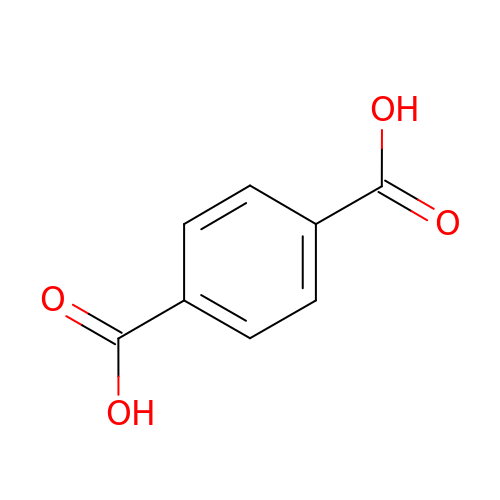terephthalic acid | C8 H6 O4 | KKEYFWRCBNTPAC-UHFFFAOYSA-N>[12x]SNALESRRAAVRAWGDQPIHLADPD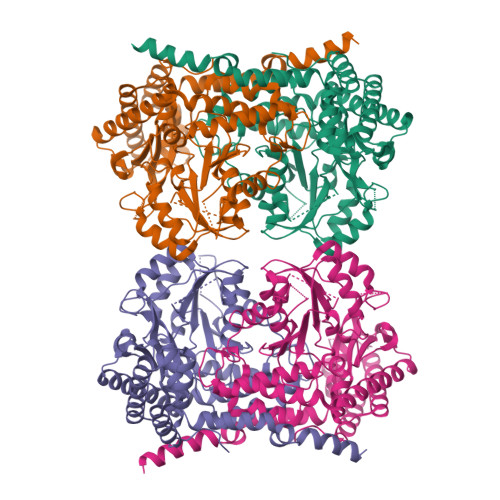IHELMEKEKQRQVRGIELIASENFVCRAVMEALGSHLTNKYSEGMPGARYYTGNQYIDQIENLCIERALTAFGLESDKWGVNVQPYSCTSANFAVYTGLLLPGERIMGLDSPSGGHMSHGYCTPGGKKISAASIFFESFPYKVNPQTGYIDYDKLEDKALDYRPKILICGGSSYPRDWDFARVRQIADKCGAVLMCDMAHISGLVATKECSNPFDHCDIVTSTTHKGLRGPRGGIIFYRRGPKIRKQGHHSSHCDTSTHYDLEEKINFAVFPSLQGGPHNNHIAALAIALKQVATPEYKAYIQQMKKNAQALAAALLRRKCRLVTGGTDNHLLLWDLTPMGLTGKVYEKVCEMCHITLNKTAIFGDNGTISPGGVRIGTPAMTTRGCIESDFETMADFLIKAAQITSALQREHGKSHKEFVKSLCTNKDIAELRNRVEAFALQYEMPASLIRIE Methanothermococcus thermolithotrophicus is the only known methanogen that grows on sulfate as its sole sulfur source, uniquely uniting methanogenesis and sulfate reduction. Here we use physiological, biochemical and structural analyses to provide a snapshot of the complete sulfate reduction pathway of this methanogenic archaeon. M. thermolithotrophicus activates SO42− by conventional ATPS and APSK, but transforms it further by uncanonical enzymes.

Inside the cell, SO42− is activated by an ATP sulfurylase (ATPS) to generate adenosine 5′-phosphosulfate (APS). The structure of MtATPS was refined to 1.97 Å resolution and obtained in an apo state despite co-crystallization with APS and SO42−. The structure exhibits the typical ATPS fold comprising three domains (domain I, 1–156; domain II, 164–314 and domain III, 320–382). Similar to many thermophilic bacteria and archaea, the domain III contains a zinc-binding domain (320–343) that might contribute to thermal stability. MtATPS superposition with structural homologues shows a slight domain rearrangement probably due to the absence of substrate. All residues critical for the reaction are conserved in MtATPS, arguing for a conserved reaction mechanism.

> GSHMVSKPHGGKLVNRVATEKTKEKILEEQNEFSKVQIREGTAIDLENIAHGVYSPLTGFLRKDEFQSVLDNMRLPNELPWSIPIVLDVTEKEKNFGEGDVILLYYNDTPIAKMQVDEIYTYDKKEFAKKVFKTDEEAHPGVAKTYALGEYLVGGEIELLNEVPNPFKSHTLRPVETRALFKEKGWETIVAFQTRNVPHLGHEYLQKLALTFVDGVFVNPVIGKKKKGDYKDEVILKAYETLFEHYYPKDTDILATVRYEMRYAGPREAIHHAIMRKNFGCTHFIVGRDHAGVGDYYGPYEAQEIFQNFPDLEISPIFFREFYYCKKCNAIVHDRICPHTSEYREHFSGTKIRNMIVNGELPPEYFMRKEVYETIRSFENPFVDE> GGSVRHIAIPAHRGLITDRNGEPLAVST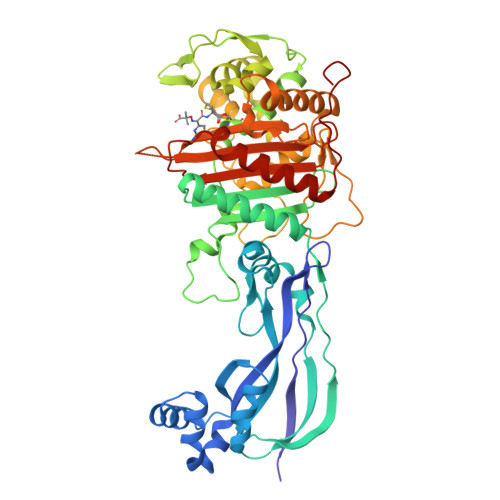PVTTLWANPKELMTAKERWPQLAAALGQDTKLFADRIEQNAEREFIYLVRGLTPEQGEGVIALKVPGVYSIEEFRRFYPAGEVVAHAVGFTDVDDRGREGIELAFDEWLAGVPGKRQVLKDRRGRVIKDVQVTKNAKPGKTLALSIDLRLQYLAHRELRNALLENGAKAGSLVIMDVKTGEILAMTNQPTYNPNNRRNLQPAAMRNRAMIDVFEPGSTVKPFSMSAALASGRWKPSDIVDVYPGTLQIGRYTIRDVSRNSRQLDLTGILIKSSNVGISKIAFDIGAESIYSVMQQVGLGQDTGLGFPGERVGNLPNHRKWPKAETATLAYGYGLSVTAIQLAHAYAALANDGKSVPLSMTRVDRVPDGVQVISPEVASTVQGMLQQVVEAQGGVFRAQVPGYHAAGKSGTARKVSVGTKGYRENAYRSLFAGFAPATDPRIAMVVVIDEPSKAGYFGGLVSAPVFSKVMAGALRLMNVPPDNLPTEFEA> MHHHHHHLILAPMVRVGTLPMRLLALDYGADIVYCEELIDLKMIQCKRVVNEVLSTVDFVAPDDRVVFRTCEREQNRVVFQMGTSDAERALAVARLVENDVAGIDVNMGCPKQYSTKGGMGAALLSDPDKIEKILSTLVKGTRRPVTCKIRILPSLEDTLSLVKRIERTGIAAIAVHGRKREERPQHPVSCEVIKAIADTLSIPVIANGGSHDHIQQYSDIEDFRQATAASSVMVARAAMWN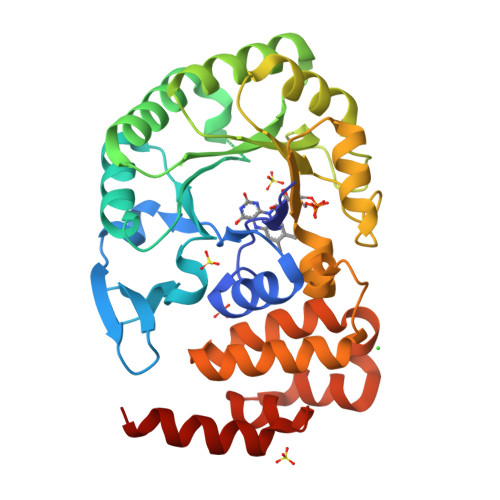PSIFLKEGLRPLEEVMQKYIRYAVQYDNHYTNTKYCLCQMLREQLESPQGRLLHAAQSSREICEAFGLGAFYEETTQELDAQQAR> LLDFDILTNDGTHRNMKLLIDLKNIFSRQLPKMPKEYIVKLVF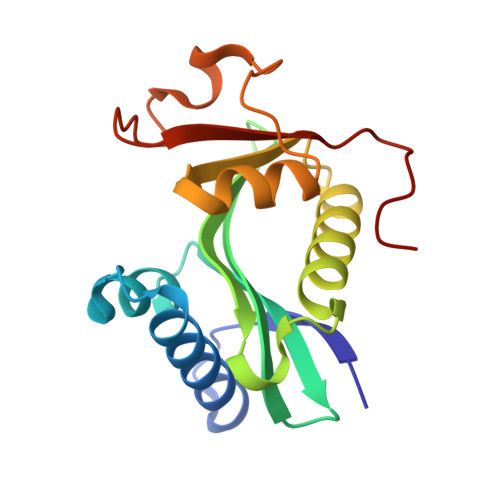DRHHESMVILKNKQKVIGGICFRQYKPQRFAEVAFLAVTANEQVRGYGTRLMNKFKDHMQKQNIEYLLTYADNFAIGYFKKQGFTKEHRMPQEKWKGYIKDYDGGTLMECYIHPYVDYGR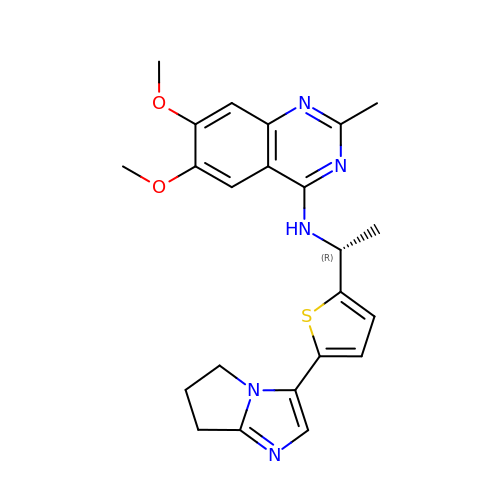~{N}-[(1~{R})-1-[5-(6,7-dihydro-5~{H}-pyrrolo[1,2-a]imidazol-3-yl)thiophen-2-yl]ethyl]-6,7-dimethoxy-2-methyl-quinazolin-4-amine | C23 H25 N5 O2 S | XRGDXPBYPNBGJI-CYBMUJFWSA-N>[2x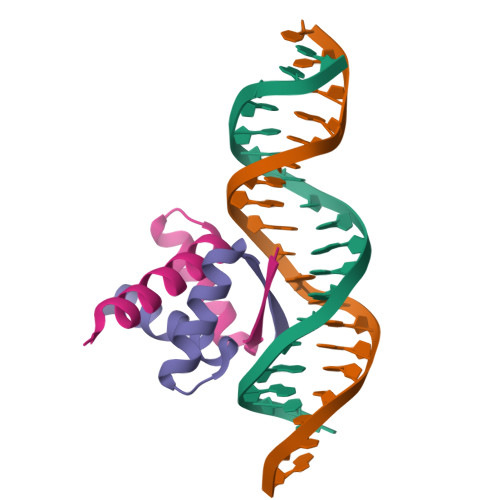]GHMGTTTMGVKLDDATRERIKSAATRIDRTPHWLIKQAIFSYLEQLENSDTLPE> MGSSHHHHHHSSGLVPRGSHMTSKTTTTVKKTSKKRATPKKNLVIVESPAKAKTIEKYLGRSYKVVASVGHIRDLKKSSMSIDFDNNYEPQYINIRGKGPLINSLKKEAKNAKQIFLASDPDREGEAISWHLAHILDLDLKGKNRVVFNEITKDAVKNAFVEPRQIDMDLVDAQQ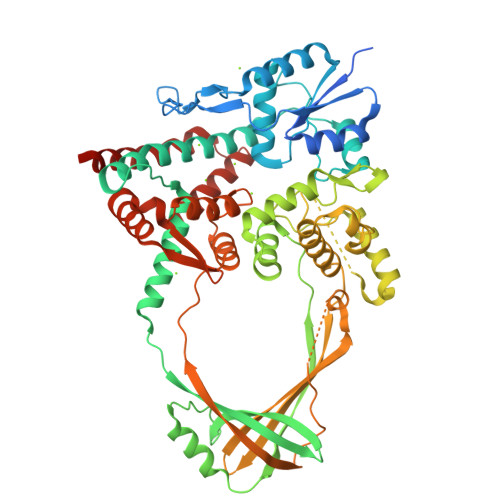ARRVLDRIVGYSISPILWKKVKKGLSAGRVQSVALKLIIDRENEIKAFKPEEYWSIDGFFKKGNKKFQANFYGLDNKKTKLKSNDDVKKVLTRIKNDDFLVDKVEKKERKRNAPLPYTTSSLQQDAANKINFRTRKTMMVAQQLYEGIRLGSNGQQGLITYMRTDSTRISPVAQNDAANYITEHFGAEYSKHGNHVRNASGAQDAHEAIRPSNVNHTPESIAKYLDKDQLKLYTLIWNRFVASQMTAAVFDTVKVNLTQNGVLFIANGSQIKFKGYMAVYNDSDKTKVLPEMIKGETVKKISANPEQHFTQPPARYSEASLIKTLEENGVGRPSTYAPTLETIQKRYYVRLVSKRFEPTELGEIVNSLIIEFFPDIVDVKFTAEMESKLDEVEIGKEEWQKVIDQFYKPFEKEVIKAEEQ>[2x]AKKIGLFYGTQTGKTESVAEIIRDEFGNDV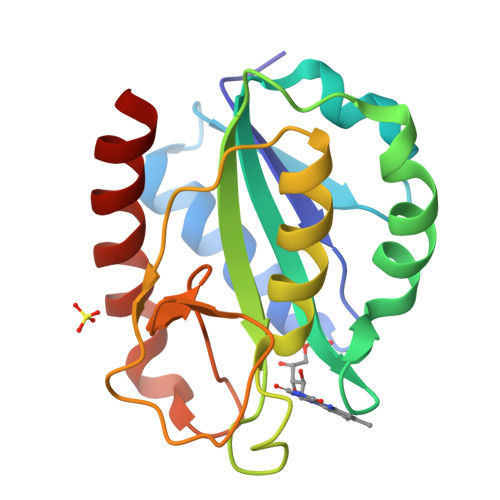VTLHDVSQAEVTDLNDYQYLIIGCPTLNIGELQSDWEGLYSELDDVDFNGKLVAYFGTGDQIGYADNFQDAIGILEEKISQRGGKTVGYWSTDGYDFNDSKALRNGKFVGLALDEDNQSDLTDDRIKSWVAQLKSEFGL> GAMAKVQVNNVVVLDNPSPFYNPFQFEITFECIEDLSED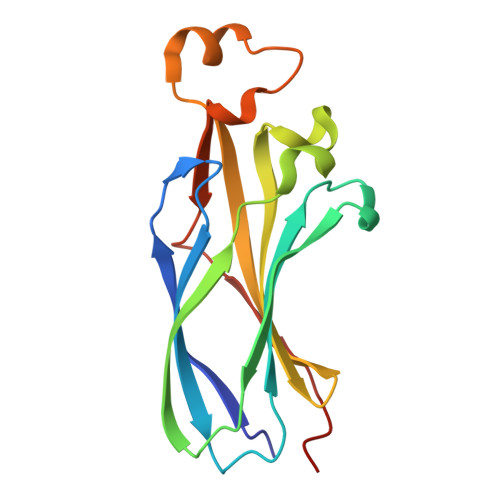LEWKIIYVGSAESEEYDQVLDSVLVGPVPAGRHMFVFQADAPNPGLIPDADAVGVTVVLITCTYRGQEFIRVGYYVNNEYTETELRENPPVKPDFSKLQRNILASNPRVTRFHINWEDN(4R)-6-(3-cyclopropyl-1-methyl-1H-indazol-5-yl)-4-methyl-1,3,4,5-tetrahydro-2H-1,5-benzodiazepin-2-one 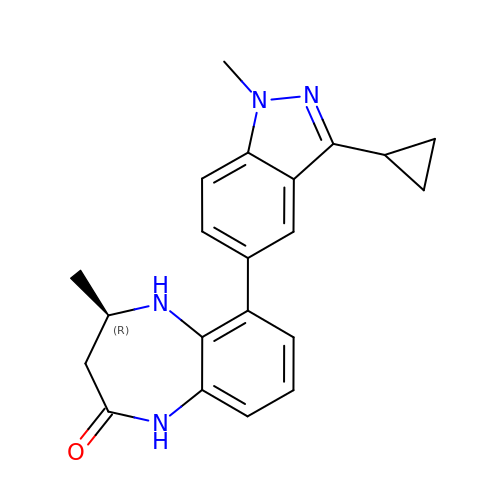| C21 H22 N4 O | RUOHSEWJRWMCPQ-GFCCVEGCSA-N>[2x]MNQSVSSLAEKDIQYQLHPYTNARLHQELGPLIIERGQGIYVYDDQGKGYIEAMAGLWSVALGFSNQRLIKAAEQQFNTLPFYHLFNHKSHRPSIELAEKLIEMAPVPMSKVFFTNSGSEANDTVVKFVWYLNNALGKPAKKKFISRVNGYHGVTVASASLTGLPGNQRGFDLPLPGFLHVGCPHHYRFA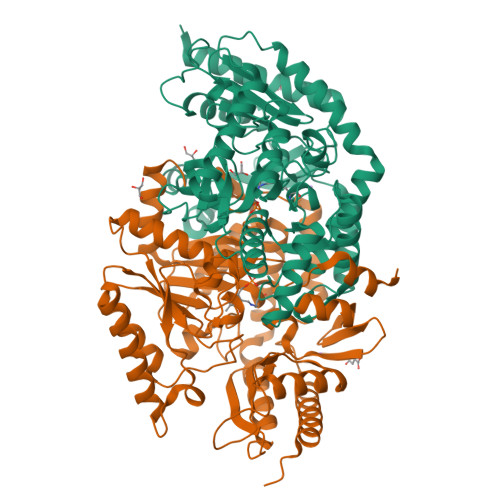LAGESEEHFADRLAVELEQKILAEGPETIAAFIGEPLMGAGGVIVPPRTYWEKIQKVCRKYDILVIADEVICGFGRTGQMFGSQTFGIQPDIMVLSKQLSSSYQPIAAILINAPVFEGIADQSQALGALGHGFTGSGHPVATAVALENLKIIEEESLVEHAAQMGQLLRSGLQHFIDHPLVGEIRGCGLIAAVELVGDRVSKAPYQALGTLGRYMAGRAQEHGMITRAMGDAVAFCPPLIVNEQEVGMIVERFARALDDTTQWVGPGG1-deoxy-2-O-phosphono-alpha-D-gluco-hept-2-ulopyranose 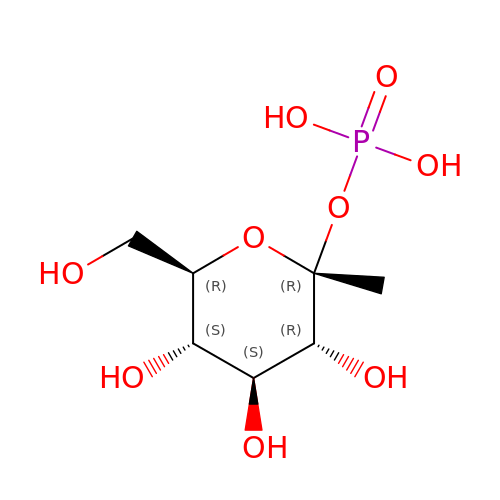| C7 H15 O9 P | QZBAZODTRUGOQS-XUUWZHRGSA-N> AMGKCPTKVVLLRNMVGAGEVDEDLEVETKEECEKYGKVGKCVIFEIPGAPDDEAVRIFLEFER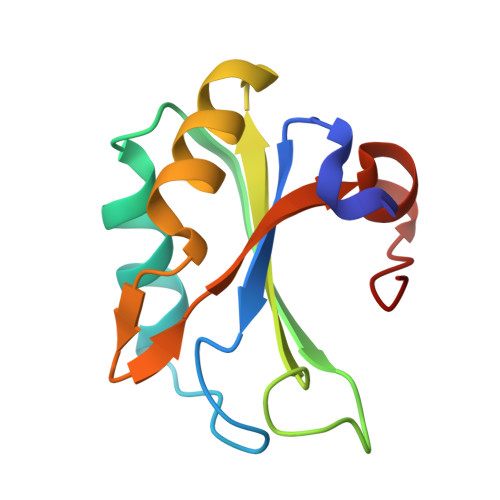VESAIKAVVDLNGRYFGGRVVKACFYNLDKFRVLDLAEQ> TIPHLAIDPFSLDFFDDPYPDQQTLRDAGPVVYLDKWNVYGVARYAEVHAVLNDPTTFCSSRGVGLSDFKKEKPWRPPSLILEADPPAHTRPRAVLSKVLSPATMKTIRDGFAAAADAKVDELLQRGCIDAIADLAEAYPLSVFPDAMGLKQEGREHLLPYAGLVFNAFGPPNELRQTAIERSAPHQAYVNEQCQRPNLAPGGFGACIHAFTDTGEITPDEAPLLVRSLLSAGLDATVNGIGAAVYCLARFPGELQRLRSD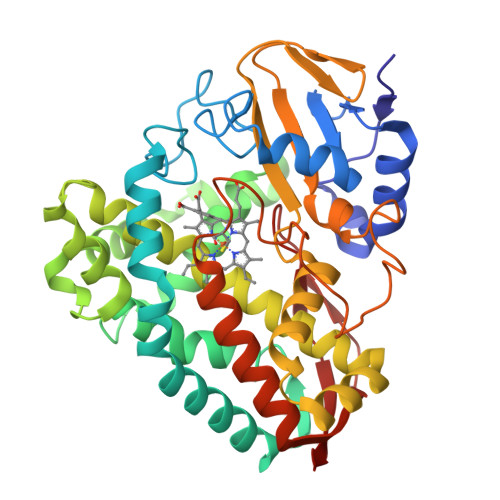PTLARNAFEEAVRFESPVQTFFRTTTREVELGGAVIGEGEKVLMFLGSANRDPRRWSDPDLYDITRKTSGHVGFGSGVHMCVGQLVARLEGEVMLSALARKVAAIDIDGPVKRRFNNTLRGLESLPVKLTPA> MNLMTTITGVVLAGGKARAMGGVDKGLLELNGKPLWQHVADALMTQLSHVVVNANRHQEIYQASGLKVIEDSLADYPGPLAGMLSVMQQEAGEWFLFCPCDTPYIPPDLAAR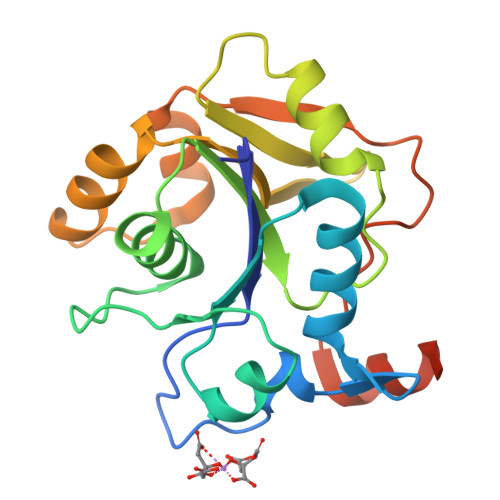LNHQRKDAPVVWVHDGERDHPTIALVNRAIEPLLLEYLQAGERRVMVFMRLAGGHAVDFSDHKDAFVNVNTPEELARWQEKRSHHHHHH4-[3-(2-Chloro-4,5-difluoro-benzoyl)ureido]-3-trifluoromethoxybenzoic acid | C16 H8 Cl F5 N2 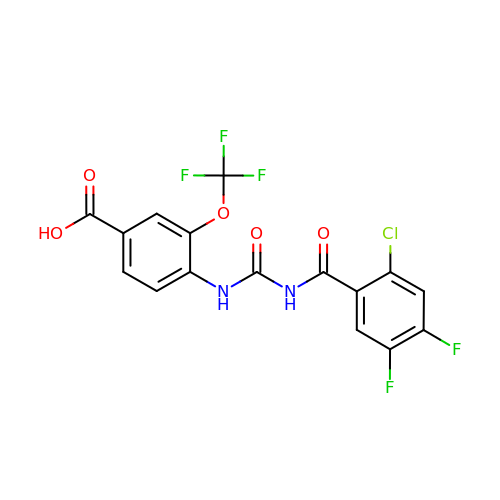O5 | NWQGDIBCFLDHDO-UHFFFAOYSA-N>[2x]MPKPVANQEDEDPTPYLFVSLEQRRIDQSKPYDSKKSCWIPDEKEGYLLGEIKATKGDIVSVGLQGGEVR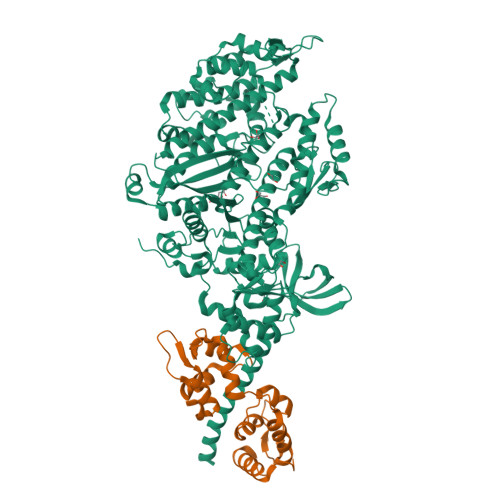DIKSEKVEKVNPPKFEKIEDMADMTVLNTPCVLHNLRQRYYAKLIYTYSGLFCVAINPYKRYPVYTNRCAKMYRGKRRNEVPPHIFAISDGAYVDMLTNHVNQSMLITGESGAGKTENTKKVIAYFATVGASKKTDEAAKSKGSLEDQVVQTNPVLEAFGNAKTVRNDNSSRFGKFIRIHFGPTGKLAGADIETYLLEKARVISQQSLERSYHIFYQIMSGSVPGVKDICLLTDNIYDYHIVSQGKVTVASIDDAEEFSLTDQAFDILGFTKQEKEDVYRITAAVMHMGGMKFKQRGREEQAEQDGEEEGGRVSKLFGCDTAELYKNLLKPRIKVGNEFVTQGRNVQQVTNSIGALCKGVFDRLFKWLVKKCNETLDTQQKRQHFIGVLDIAGFEIFEYNGFEQLCINFTNEKLQQFFNHHMFVLEQEEYKREGIDWAFIDFGMDLLACIDLIEKPMGILSILEEESMFPKATDQTFSEKLTNTHLGKSAPFQKPKPPKPGQQAAHFAIAHYAGCVSYNITGWLEKNKDPLNDTVVDQFKKSQNKLLIEIFADHAGQSGGGEQAKGGRGKKGGGFATVSSAYKEQLNSLMTTLRSTQPHFVRCIIPNEMKQPGVVDAHLVMHQLTCNGVLEGIRICRKGFPNRMMYPDFKMRYQILNPKGIKGIEDPKKCTKVLIESTELNDDQYRLGNTKVFFRAGVLGQMEEFRDERLGKIMSWMQAWARGYLSRKGFKKLQEQRVAL;>[2x]MADVPKREVENVEFVFEVMGSPGEGIDAVDLGDALRALNLNPTLALIEKLGGTKKRNEKKIKLDEFLPIYSQVKKEKEQGCYEDFIECLKLYDKEENGTMLLAELQHALLALGESLDDEQVETLFADCMDPEDDEGFIPYSPFLARMCDRPDQLK>[60x]MSTFLDSFEEWYETAAASWRNLKAGAPQPKPNQQSQSVSPDREPERKDNNRGFVLPGYKYLGPGNGLDKGPPVNKADSVALEHDKAYDQQLKAGDNPYIKFNHADQDFIDSLQDDQSFGGNLGKAVFQAKKRILEPFGLVEDPVNTAPAKKNTGKLTDHYPVVKKPKLTEEVSAGGGSSAVQDGGATAEGTEPVAASEMAEGGGGAMGDSSGGADGVGNASGNWHCDSQWMGNTVITKTTRTWVLPSYNNHIYKAITSGTSQDANVQYAGYSTPWGYFDFNRFHCHFSPRDWQRLINNHWGIRPKSLKFKIFNVQVKEVTTQDQTKTIANNLTSTIQVFTDDEHQLPYVLGSATEGTMPPFPSDVYALPQYGYCTMHTNQNGARFNDRSAFYCLEYFPSQMLRTGNNFEFTFDFEEVPFHSMFAHSQDLDRLMNPLVDQYLWNFNEVDSSRNAQFKKAVKGAYGTMGRNWLPGPKFLDQRVRAYTGGTDNYANWNIWSNGNKVNLKDRQYLLQPGPVSATYTEGEASSLPAQNILGIAKDPYRSGSTTAGISDIMVTEEQEVAPTNGVGWKPYGRTVTNEQNTTTAPTSSDLDVLGALPGMVWQNRDIYLQGPIWAKIPKTDGKFHPSPNLGGFGLHNPPPQVFIKNTPVPADPPVEYVHQKWNSYITQYSTGQCTVEMVWELRKENSKRWNPEIQFTSNFSNRTSIMFAPNETGGYVEDRLIGTRYLTQNL

Goose parvovirus (GPV) is a member of Parvoviridae, a family of non-enveloped single-stranded DNA (ssDNA) viruses with T = 1 icosahedral capsids. Adeno-associated viruses (AAVs) are also in this genus, which are widely used as vectors for gene therapy applications. It is noteworthy to mention that few dependoparvoviruses, such as GPV and Muscovy duck parvovirus (MDPV), are pathogenic and do not require coinfection with a helper virus to replicate in host cells. On the other hand, the “right” ORF expresses the three capsid viral proteins (VPs), VP1 (81 kDa), VP2 (65 kDa), and VP3 (60 kDa), that assemble the icosahedral capsid, with VP3 being the major capsid protein. Goose parvovirus (GPV) is an etiological agent of Derzsy’s disease, afflicting geese and Muscovy ducks worldwide.

The Bac-to-Bac® baculovirus expression system was used to produce VLPs of GPV comprised of VP3 exclusively. From these micrographs, capsid images were used to reconstruct a 3D GPV capsid structure with a final resolution of 2.43 Å. The GPV capsid structure shows surface morphologies generally conserved among parvoviruses, including five-fold channels, three-fold protrusions, two-fold depressions, and two/three-fold walls. The beginning of structural ordering at the N-terminus was observed at alanine 214, which is similar to most AAV VP structures determined to date. Following alanine 214, the VP3 amino acid side chain densities were well ordered to leucine 732 at the C-terminus. The overall GPV VP structure conserves the core β-strand A, the eight-stranded anti-parallel β-barrel (βB-βI), and the α-helix A, as well as the general positioning of the surface loops. Significant differences were observed in several variable regions, including VR-III, VR-IV, VR-V, and VR-VII. GPV has the largest VR-III loop, which is a result of AAV5, AAV2, and QAAV possessing one, two, or three amino acid deletions in the corresponding region, respectively. In short, GPV may not interact with SIA nor HSPG for transduction initiation, and it is unlikely that the GPV capsid binds to AAVR. Monomer alignments of GPV, QAAV, AAV2, and AAV5 show that the DE and HI loops (which form the five-fold region) of GPV have very similar conformations, which explains its mAb 2–7 recognition.>[2x]QQASTLPDLAEQFAPPDVAPPLLIKLVEAIEKKGLECSTLYRTQSSSNPAELRQLLDCDTASLDLEMFDVHVLADAFKRYLLDLPNPVIPVAVSSELISLAPEVQSSEEYIQLLKKLIRSPSIPHQYWLTLQYLLKHFFKLSQTSSKNLLNATVLSELFSPLLFRFPAASSENTEHLIKIIEILISTEWNERQ

The N-terminal domains of p85α include an SH3 domain, capable of binding to proline-rich sequences, and a BH (breakpoint cluster region homology) domain. The BH domain can bind to and regulate several GTPases including Rab5, Rac1 and Cdc42. In addition, the p85α BH domain, either alone or together with the SH3 domain, can bind to and positively regulate PTEN activity. The p85α BH domain also exhibits Rab5 GAP activity to stimulate Rab5-mediated GTP hydrolysis required to inactivate Rab5-mediated protein trafficking functions.

To determine if the patient-derived p85α BH domain mutations impacted the overall folded structure of the BH domain, several of these BH domain mutants were crystalized and their structures were determined using X-ray crystallography. X-ray diffraction data collection and structure refinement statistics for bovine p85α (105–319) mutants (E137K, E217K, R262T, E297K) are provided in Supplementary Table S1. In contrast, the bladder cancer-associated p85α mutants, E137K and R262T, showed a slightly enhanced Rab5 binding. Several patient-derived mutations within the BH domain of p85α can enhance PTEN binding (e.g. R262T) that may help to stabilize PTEN by blocking its ubiquitination. Further, crystal structure determinations for several of these mutant BH domains indicated that no major structural alterations were present. No significant differences in protein flexibility were observed for any of the mutant proteins, suggesting that the mutations did not alter the rigidity of the domain.>[2x]SARVGSQNGVQMLSPSEIPQRDWFPSDFTFGAATSAYQIEGAWNEDGKGESNWDHFCHNHPERILDGSNSDIGANSYHMYKTDVRLLKEMGMDAYRFSISWPRILPKGTKEGGINPDGIKYYRNLINLLLENGIEPYVTIFHWDVPQALEEKYGGFLDKSHKSIVEDYTYFAKVCFDNFGDKVKNWLTFNDPQTFTSFSYGTGVFAPGRCSPGLDCAYPTGNSLVEPYTAGHNILLAHAEAVDLYNK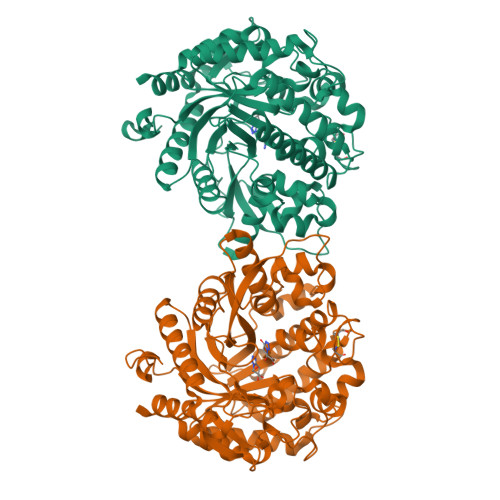HYKRDDTRIGLAFDVMGRVPYGTSFLDKQAEERSWDINLGWFLEPVVRGDYPFSMRSLARERLPFFKDEQKEKLAGSYNMLGLNYYTSRFSKNIDISPNYSPVLNTDDAYASQEVNGPDGKPIGPPMGNPWIYMYPEGLKDLLMIMKNKYGNPPIYITENGIGDVDTKETPLPMEAALNDYKRLDYIQRHIATLKESIDLGSNVQGYFAWSLLDNFEWFAGFTERYGIVYVDRNNNCTRYMKESAKWLKEFNTAKKPSKKILTPA> MMSREADHTIKGFLYQFNKTLNSILSSTDQDEIQIEGIIEDIDIKNSNITNAIQCKYHESKVRHNLSDIYKPILQMLLHFLENDSLNIKYALYAYFPNEQVGVKEVTKSQIEEILSSSNFDYISKYISKIKPPKEQIIKELLGKTSKTTEDKTRIKKYYETSKLE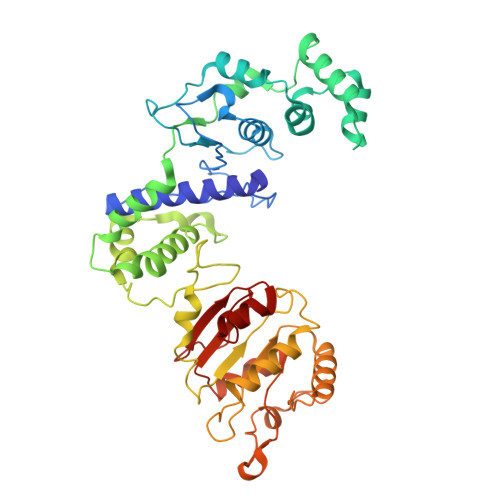TIVDIDKFLRDHFVFEIGLSYEELMNETKNLLMKEGFSLEDVKDLFYPNSIQYIAELSILPEAEKRISSKNKLIDYLKGNKKTAMSRWTSEVLTRKQLLKVRKNQLVPSLNINSRSRYFIIDPDTIDNFDDEFILFVKDYLDKYNSKIKLHTETPCFILKTDVNNLSEYHKRFVSRNIQIITGYIGDTFYFKEFNKEPKRIIKDNWVEFKARISCNSDEVIKCINYKKCDDLYIVGGVDVSLLDTADVNIENLEINNFRELKYLLSMLKEI> MEPKVAELKQKIEDTLCPFGFEVYPFQVAWYNELLPPAFHLPLPGPTLAFLVLSTPAMFDRALKPFLQSCHLRMLTDPVDQCVAYHLGRVRESLPELQIEIIADYEVHPNRRPKILAQTAAHVAGAAYYYQRQDVEADPWGNQRISGVCIHPRFGGWFAIRGVVLLPGIEVPDLPPRKPHDCVPTRADRIALLEGFNFHWRDWTYRDAVTPQERYSEEQKAYFSTPPAQRLALLGLAQPSEKP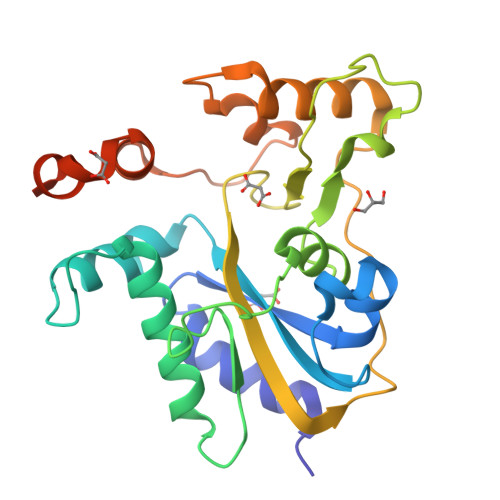SLEHHHHHH Structurally, talin contains an N-terminal FERM domain (F0-F3) linked to 13 helical bundles (rod region, R1-R13) terminating in a dimerization domain (DD). The FERM domain binds and activates integrins, while the rod region contains vinculin-binding sites and actin-binding sites that couple integrins to the actomyosin machinery. Tensin3 consists of an N-terminal PTEN homology domain, a large intrinsically disordered region (IDR), and C-terminal SH2 and PTB domains. An exception is a talin-binding site (TBS) in the IDR, which is critical for FB formation and FN fibrillogenesis.

We first determined the structure of the talin–R11R12 in complex with tensin3 TBS to 2.76 Å resolution. This revealed that the tensin3 TBS forms an amphipathic α-helix that binds between the α2-α5 helices of the R11 bundle, forming a 6-helix bundle. Residues D696, S698, and D710 on tensin3 TBS establish electrostatic contacts with K2024, K2119, and K2133 on R11, while K2031 orients its sidechain away from L705 on tensin3. The hydrophobic surface of R11 engages with the uncharged face of TBS, with tensin3 residues L702 and I706 forming the core of the hydrophobic interface, demonstrating that these sites are critical for tensin3 interaction with talin R11. The R11-TBS structure demonstrated that the positively charged residues K2024 and K2031 on talin are involved in R11 binding to tensin3 TBS. However, the double mutation (K2024E+K2031E), referred to hereafter as the “R11m” mutant, completely abolished the recruitment. We therefore modeled the complexes using AlphaFold3 and low-quality electron density, which supports the general location and orientation of the helix on R7R8. This approach is justified by comparing the predicted structure and our experimental structure of the R11R12–tensin3 TBS complex, which are almost identical. Determining the structure of the tensin3 TBS in complex with talin R11R12 enabled us to design a point mutation (L702E) in tensin3 that completely disrupted its interaction with talin. Thus, L702 is critical for tensin3 interactions with all binding sites in talin, and these interactions share a similar mechanism. Talin R7R8 is characterized with the lowest Kd (15.8 ± 0.9 μM), with an enthalpy of 42.72 ± 2.06 kJ/mol. These endothermic binding profiles are similar to our previous observation regarding talin R11 with tensin3 TBS (17 μM).

>[2x]GTFTGIDPFTGTQACITAASAVSGIIADLDTTIMFATAGTLNREGAETFADHREGILKTAKVLVEDTKVLVQNAAGSQEKLAQAAQSSVATITRLADVVKLGAASLGAEDPETQVVLINAVKDVAKALGDLISATKAAAGKVGDDPAVWQLKNSAKVMVTNVTSLLKTVKAVEDEATKGTRALEATTEHIRQELAVFCSPEPPAKTSTPEDFIRMTKGITMATAKAVAAGNSCRQEDVIATANLSRRAIADMLRACKEAAFHPEVAPDVRLRALHYGRECANGYLELLDHVLLTLQKPNPDLKQQLTGHSKRVAGSVTELIQAAEAMKGT;>[2x]TLDIDQSIEQLNRLILELDPTFEPIPT(2R,4S)-N-butyl-4-[(5S,8S,10R)-5,10-dimethyl-3,3,6-trioxo-3lambda~6~-thia-7-azabicyclo[11.3.1]heptadeca-1(17),13,15-trien-8-yl]-4-hydroxy-2-methylbutanamide | C26 H42 N2 O5 S | 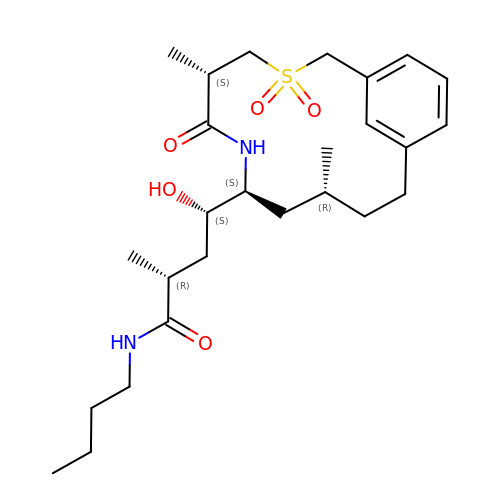RYVHNXNTYFQKLT-FSQPGOEKSA-N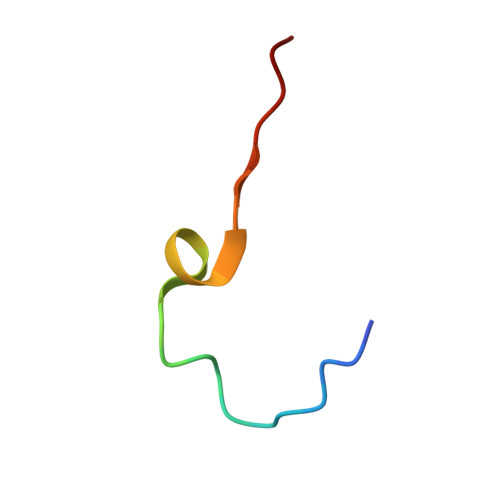> GNEGVIINNYYSNQYQNSIDLSAN>MTPSTPIDDAEIARSIALEDIDVSKPELFERDGLHPYFERLRREDPVHYCKASEYGPYWSITKFSDIVAIDTNHKVFSSDHTNGSFVLDDTTLNAVDGGIYLPNFLGMDPPKHDVHRMVVSPIVAPQNLLRFEATIRERTKRVLSELPIGEEFNWVDRVSIELTTMMLATLLDFPFDDRRKLTRWSDIITTRPGYGLVDSWEQRESELMECLAYFQRLYAERQAMPPKPDLISMLAHSPEMQDLTPTDFLGTLALLIVGGNDTTRSSMSGSAMACHLY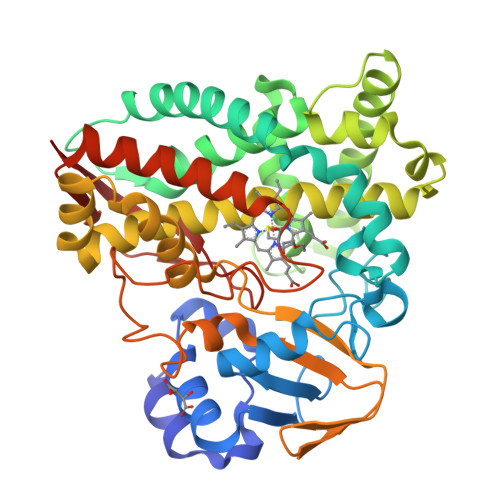PQEFDKVRNNRALLASVIPEVVRWQTPIAHMRRTALEDVEFRGKQIRKGDKVVMWYLSGNRDDEVIDRPMDFIADRPRARHHLSFGFGIHRCLGNRLAELQLKILWEEMCERYSRIEVCGEPVRVPSNLVHGYIDIPVRLHA[3x]> MTTYLEFIQQNEERDGVRFSWNVWPSSRLEATRMVVPVAALFTPLKERPDLPPIQYEPVLCSRTTCRAVLNPLCQVDYRAKLWACNFCYQRNQFPPSYAGISELNQPAELLPQFSSIEYVVLRGPQMPLIFLYVVDTCMEDEDLQALKESMQMSLSLLPPTALVGLITFGRMVQVHELGCEGISKSYVFRGTKDLSAKQLQEMLGLSKVPLTQATRGPQVQQPPPSNRFLQPVQKIDMNLTDLLGELQRDPWPVPQGKRPLRSSGVALSIAVGLLECTFPNTGARIMMFIGGPATQGPGMVVGDELKTPIRSWHDIDKDNAKYVKKGTKHFEALANRAATTGHVIDIYACALDQTGLLEMKCCPNLTGGYMVMGDSFNTSLFKQTFQRVFTKDMHGQFKMGFGGTLEIKTSREIKISGAIGPCVSLNSKGPCVSENEIGTGGTCQWKICGLSPTTTLAIYFEVVNQHNAPIPQGGRGAIQFVTQYQHSSGQRRIRVTTIARNWADAQTQIQNIAASFDQEAAAILMARLAIYRAETEEGPDVLRWLDRQLIRLCQKFGEYHKDDPSSFRFSETFSLYPQFMFHLRRSSFLQVFNNSPDESSYYRHHFMRQDLTQSLIMIQPILYAYSFSGPPEPVLLDSSSILADRILLMDTFFQILIYHGETIAQWRKSGYQDMPEYENFRHLLQAPVDDAQEILHSRFPMPRYIDTEHGGSQARFLLSKVNPSQTHNNMYAWGQESGAPILTDDVSLQVFMDHLKKLAVSSA;> EGLRVVNLLQERNMLPSTPLKPPVPNLHEDIQKLNCNPELFRCTLTSIPQTQALLNKAKLPLGLLLHPFKDLVQLPVVTSSTIVRCRSCRTYINPFVSFLDQRRWKCNLCYRVNDVPEEFLYNPLTRVYGEPHRRPEVQNATIEFMAPSEYMLRPPQPPVYLFVFDVSHNAVETGYLNSVCQSLLDNLDLLPGNTRTKIGFITFDSTIHFYGLQESLSQPQMLIVSDIEDVFIPMPENLLVNLNESKELVQDLLKTLPQMFTKTLETQSALGPALQAAFKLMSPTGGRMSVFQTQLPTLGVGALKPREEPNHRSSAKDIHMTPSTDFYKKLALDCSGQQVAVDLFLLSGQYSDLASLGCISRYSAGSVYYYPSYHHQHNPVQVQKLQKELQRYLTRKIGFEAVMRIRCTKGLSIHTFHGNFFVRSTDLLSLPNVNPDAGYAVQMSVEESLTDTQLVSFQSALLYTSSKGERRIRVHTLCLPVVSTLNDVFLGADVQAISGLLANMAVDRSMTASLSDARDALVNAVIDSLSAYRSSVLSNQQPGLMVPFSLRLFPLFVLALLKQKSFQTGTNARLDERIFAMCQVKNQPLVYLMLTTHPSLYRVDNLSDEGALNISDRTIPQPPILQLSVEKLSRDGAFLMDAGSVLMLWVGKNCTQNFLSQVLGVQNYASIPQPMTDLPELDTPESARIIAFISWLREQRPFFPILYVIADESPMKANFLQNMIEDRTESALSYYEFLLHIQQQVNK;> MVLLTMIARVADGLPLAASMQEDEQSGRDLQQYQSQAKQLFRKLNEQSPTRCTLEAGAMTFHYIIEQGVCYLVLCEAAFPKKLAFAYLEDLHSEFDEQHGKKVPTVSRPYSFIEFDTFIQKTKKLYIDSRARRNLGSINTELQDVQRIMVANIE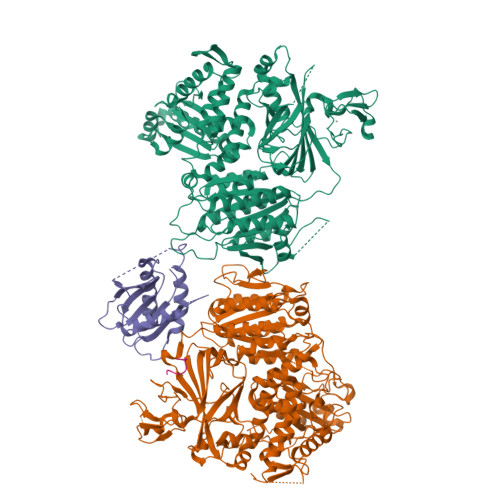EVL;> QIYTDIEMNR[4-({5-amino-3-[(4-sulfamoylphenyl)amino]-1H-1,2,4-triazole-1-carbonyl}amino)phenoxy]acetic acid | C17 H17 N7 O6 S | 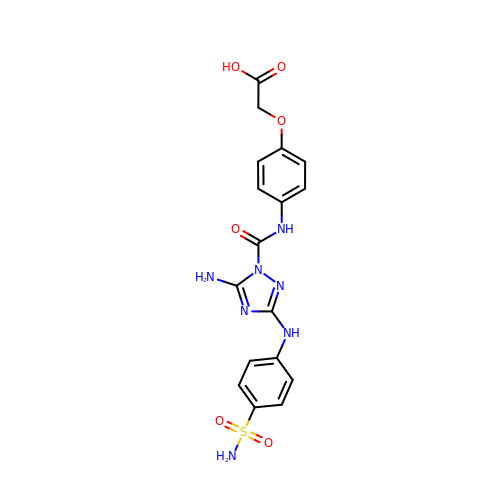QQXWNIAQCDPFCH-UHFFFAOYSA-N> IESIIKTATDTVKSEINAELGVVPSLNAVETGASSNTEPEEAIQTRTVINQHGVSETLVENFLSRAALVSKRSFEYKNHTSSEARTDKNFYKWTINTKSFVQLRRKLELFTYLRFDAEITILTTVAVGSNNSTYMGLPDLTLQAMFVPTGALTPEKQDSFHWQSGSNASVFFKVSDPPARMTIPFMCINSAYSVFYDGFAGFEKNGLYGINPADTIGNLCVRIVNEHQPIGFTVTVRVYMKPKHIKAWAPRPPRTLPYMSIANANYKGKERAPNALNAIIGNRESVKTMPHDIVLV;> SPSAEACGYSDRVLQLKLGNSAIVTQEAANYCCAYGEWPNYLPDHEAVAIDKPTQPETATDRFYTLKSVKWETESTGWWWKLPDALNNIGMFGQNVQHHYLYRSGFLIHVQCNATKFHQGALLVVAIPEHQRGAHNTTTSPGFDDIMKGEEGGTFNHPYVLDDGTSLACATIFPHQWINLRTNNSATIVLPWMNAAPMDFPLRHNQWTLAIIPVVPL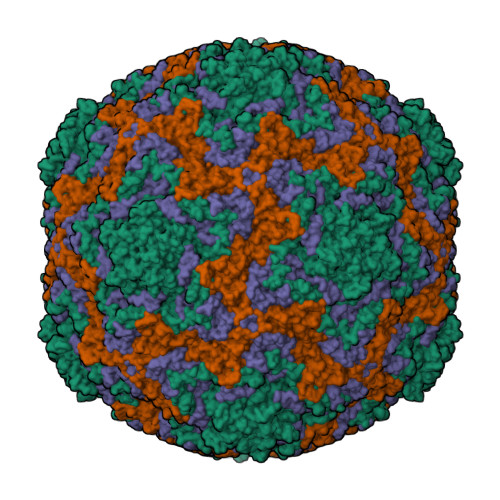GTRTVSSMVPITVSIAPMCCEFNGLRHAITQ;> GVPTYLLPGSGQFLTTDDHSSAPVLPCFNPTPEMHIPGQVRNMLEVIQVESMMEINNTENAVGMQRLKVDISVLTDVDQLLFNIPLDIQLDGPLRNTLVGNISRYYTHWSGSLEMTFMFCGSFMATGKLILCYTPPGGSCPTTRETAMLGTHIVWDFGLQSSVTLVIPWISGSHYRMFNNDAKSTNANVGYVTCFMQTNLIVPSESSNTCSLIGFVAAKDDFSLRLMRDSPDIGQLEHLHEAEAAYQ;> MGAQVTRQQTGTHENANIATNGSHITYNQINFYKDSYAASASKQDFSQDPSKFTEPVVEGLKAGAPVLK>MSTKKPNEIVITKSKRIEDYVLDTIILFNQGYEEVEIRGSGQEINKAIEVYNQLVDRLKEGVRLEKVDIGSEVKDRRRISYI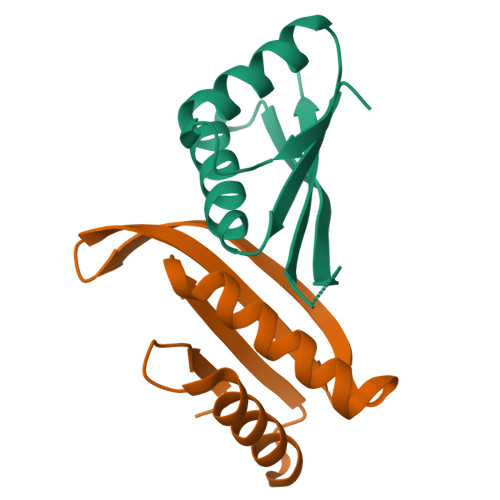LLRLKRIY[3x]Amyloid-β (Aβ) forms heterogeneous oligomers, which are implicated in the pathogenesis of Alzheimer’s disease (AD). Peptides Aβm17–36 and Aβm17–35 mimic two different β-hairpins that Aβ can form, the Aβ17–36 and Aβ17–35 β-hairpins, respectively. These hairpins are similar in composition but differ in hairpin alignment, altering the facial arrangements of the side chains of the residues that they contain. Aβm17–36 and Aβm17–35 are cyclic hexadecapeptides consisting of two heptapeptide β-strands (Aβ17–23 and Aβ30–36 or Aβ29–35) connected by two δ-linked ornithine turn units that promote a β-hairpin-like conformation.

Aβm17–36 is designed to display the side chains of Val36, Leu34, Ile32, and Ala30 on the same face of the β-hairpin as the side chains of Leu17, Phe19, Ala21, and Asp23 (the LFAD face). The X-ray crystallographic phases of Aβm17–36 were solved by soaking the crystals in potassium iodide to incorporate iodide ions into the crystal lattice and then performing single-wavelength anomalous diffraction (SAD) phasing. The X-ray crystallographic structure of Aβm17–36 contains 16 molecules of Aβm17–36 in the asymmetric unit. Each of the molecules folds to form a twisted β-hairpin, and variation between monomers is minimal, consisting mainly of Met35 and Leu34 rotamers. The trimers formed by Aβm17–36 consist of three β-hairpins in a triangular assembly with a cavity at the center of the triangle. Phe20 and Phe19 sit on opposite faces at the center of the trimer surrounding this cavity. The trimer is stabilized by hydrophobic packing of residues on both faces and by intermolecular hydrogen bonding between the backbones of Val18 and Glu22 at each corner. Two trimers further pack together on the VFE face to form a hexamer. Although the hexamer is not stabilized by hydrogen bonds between the component trimers, it is stabilized by bridging water molecules that hydrogen bond to both trimers. The side chains of residues Phe20, Glu22, and Ile31 form the hydrophobic core of the hexamer, with the carboxyl groups of Glu22 sitting at the corners.

>[16x]ALVFFAEDAAIIGLMV> GMLTDMQRDSASSSTVTTEQIVYGALPLTTINEPECRAIAITSINGSATLSGVSGPMGDQTDADLLIQLRGWADAIVVGAETARKENYGPVVLP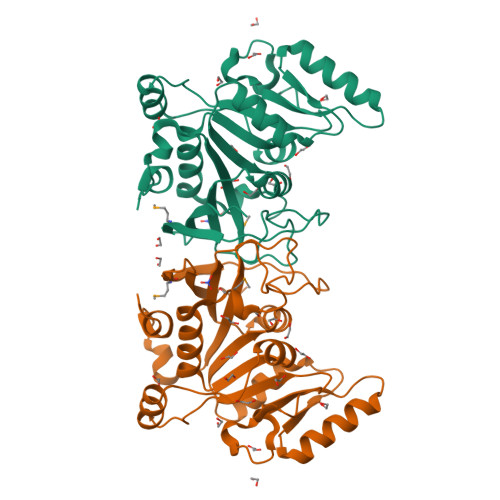HGIKNQRQKLGRCGLPKLTLLSKSLYFDFSSELFSPDLPSELSPLVITQQPANNSEQWDQRLQKLIDVGVEVIVAPTSTNPLKIAFDALHARRLKKISIEGGPSVYRQALSLGIVDRLHLTIAPNIICPVESPLFGKISDDSFTTRLVLEMLSSSPNGLIFSRYKVIRDTLGNPTQ>[2x]CG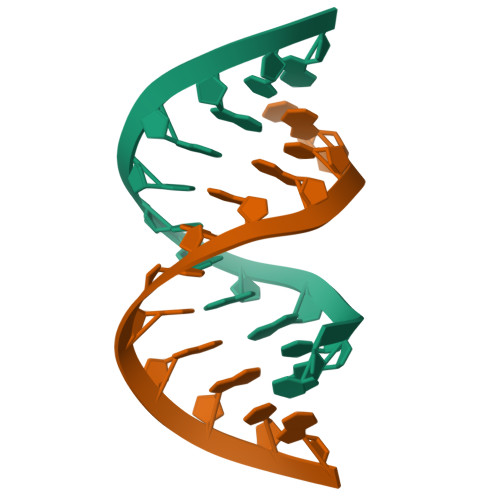CGAAUUAGCG> CRIHEISCGAHSTQCIPVSWRC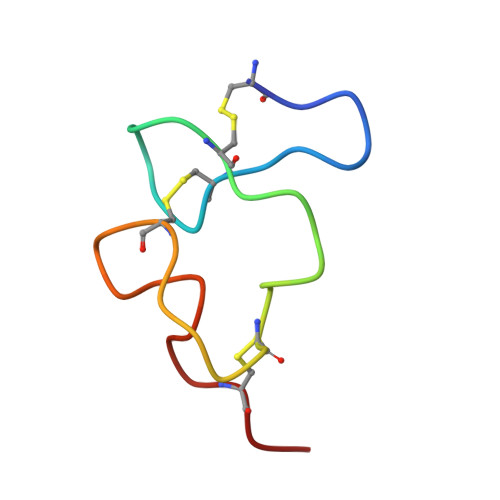DGENDCDSGEDEENCGN>GPLGSEERESELSSNPAASAGASLEPPAAPAPGEDNPAGAGGAAVAGAAGGARRFLCGVVEGFYGRPWVMEQRKELFRRLQKWELNTYLYAPKDDYKHRMFWREMYSVEEAEQLMTLISAAREYEIEFIYAISPGLDITFSNPKEVSTLKRKLDQVSQFGCRSFALLFDDIDHNMCAADKEVFSSFAHAQVSITNEIYQYLGEPETFLFCPTEYCGTFCYPNVSQSPYLRTVGEKLLPGIEVLWTGPKVVSKEIPVESIEEVSKIIKRAPVIWDNIHANDYDQKRLFLGPYKGRSTELIPRLKGVLTNPNCEFEANYVAIHTLATWYKSNMNGVRKDVVMTDSEDSTVSIQIKLENEGSDEDIETDVLYSPQMALKLALTEWLQEFGVPHQYSSRQVAHSGAKASVVDGTPLVAAGGGGSGGGGSVTLEDLQLLADLFYLPYEHGPKGAQMLREFQWLRANSSVVSVNCKGKDSEKIEEWRSRAAKFEEMCGLVMGMFTRLSNCANRTILYDMYSYVWDIKSIMSMVKSFVQWLGCRSHSSAQFLIGDQEPWAFRGGLAGEFQRLLPIDGANDLFFQPPPLTPTSKVYTIRPYFPKDEASVYKICREMYDDGVGLPFQSQPDLIGDKLVGGLLSLSLDYCFVLEDEDGICGYALGTVDVTPFIKKCKISWIPFMQEKYTKPNGDKELSEAEKIMLSFHEEQEVLPETFLANFPSLIKMDIHKKVTDPSVAKSMMACLLSSLKANGSRGAFCEVRPDDKRILEFYSKLGCFEIAKMEGFPKDVVILGRSL[2x]

Nucleocytoplasmic protein O-GlcNAcylation is a dynamic modification catalysed by O-GlcNAc transferase (OGT) and reversed by O-GlcNAc hydrolase (OGA), whose activities are regulated through largely unknown O-GlcNAc-dependent feedback mechanisms. OGA is a homodimeric, multi-domain enzyme containing a catalytic core and a pseudo-histone acetyltransferase (pHAT) domain. Here, we show that the eukaryotic OGA pHAT domain forms catalytically incompetent, symmetric homodimers, projecting a partially conserved putative peptide-binding site. In solution, OGA exist as flexible multi-domain dimers, but catalytic core-pHAT linker interactions restrict pHAT positional range.

A construct was designed that lacks the large, disordered loop (residues 397–535) while retaining the pHAT domains. As with TaOGA, this hOGA construct was expressed and purified from E. coli, imaged by cryo-EM, and processed using CryoSPARC. Both 2D and 3D classifications showed particle classes with well-defined catalytic and stalk domains, but none of these included fully defined pHAT domains. Instead, these domains appeared as blurred density in 2D and as an elongated asymmetric density between the two stalk domains in 3D, suggesting that the pHAT domains adopt a range of different angular positions relative to the catalytic core. To further explore this heterogeneity, particles were sub-classified to enrich for more populated conformations. This analysis yielded four major conformations—termed I, II, III and IV—each separately subjected to 3D reconstruction and refined to global resolutions ranging from 3.3 Å to 4.0 Å. An AlphaFold3 model of hOGA was used to guide model building, and across all conformations the catalytic core consistently displayed a near two-fold symmetry, forming two glycoside hydrolase active sites composed of the catalytic domain of one monomer and the stalk domain of the other. In all four conformations of hOGA, the cryo-EM density maps reveal a discontinuity in the region following Leu701, corresponding to the linker connecting the catalytic core and the pHAT domains. This linker (LFFQPPPLTPTSKVY) is of medium length and proline-rich, characteristics known to disrupt secondary structures and enhance conformational flexibility. In contrast, our hOGA cryo-EM structures containing the pHAT domains reveal defined, albeit at lower resolution, density for both regions, suggesting that the presence of the pHAT domains stabilises these otherwise flexible regions. Unlike the crystal structures of hOGA without pHAT domains, all four conformations display additional density in the active site. Superimposing a crystal structure of hOGA with GlcNAc in the active site suggests a density compatible with GlcNAc, presumably co-purified with the enzyme from E. coli lysates.>[14x]MAKELHFNKDMQALKRMQAGVDKLATVVGVTIGPKGRNVVLESKFGAPKIVNDGVTIAREVELSDPVENIGATLVRQAAARTNDTAGDGTTTATVLSAAFIAEGMKIVSAGTNPVQLVRGMEKTVQELVKELRKMSSVVQTDKDLANVACVSAGGNTDIGSLISDAMAKVGRTGVVTMEEGKTAEDQLVFVEGMQFERGYTSPYFVTDPERMICEYENCKILLVDKKISTARDIITILESAIRGNYPLLIMAEEVEQEALATLVVNKLRGTLKVVAIKAPGFGERRSSYLEDIAILTGGTVVRDEMGVSLEQATDAVLGTAAKITITKERTTVVGDGSTAADVAARVKQIRNLQMQTDQDYEREKLQERIARLSGGVAIIQVGAQTETELKEKKLRVEDALNATRAAVEEGVVPGGGCTLLRLSEKVDVIKRRMTDPEQQMGADIIKRALCYPIKLIAQNAGVNGSVVMNEVMKNLDRPHYGYNAATDSFENLMETGIIDPSKVVRCSMENAVSVAKTFLLADVVVTELKEIEAGAKPNPVAPGAAGFGGGL

Chloroplast chaperonin, consisting of multiple subunits, mediates folding of the highly abundant protein Rubisco with the assistance of co-chaperonins. Unlike homo-oligomeric GroEL and mitochondrial Hsp60, chloroplast chaperonin consists of multiple subunits, diverging into two distinct but related α and β types. Though the authentic chloroplast chaperonin consists of both subunit types in vivo, homo-oligomeric Cpn60β is functional in refolding model substrates with assistance from co-chaperonin in vitro. ATP hydrolysis drives the chaperonin allosteric cycle to assist substrate folding and promotes disassembly of chloroplast chaperonin.

The crystallization of functional hetero-oligomers of CPN60 did not succeed, whereas the crystallization of CPN60β1 homo-oligomers was achieved by the sandwich method. The crystals belong to space group P21, with 14 subunits per asymmetric unit. In our study, the first crystal structure of Chlamydomonas chloroplast chaperonin homo-oligomer (CPN60β1) was solved at 3.8 Å, and displayed a rigid body and structural features such as looser compaction, a larger central cavity, less contact sites, and an enlarged ATP binding pocket compared to GroEL. In overall architecture, CPN60β1 presents as a typical type I chaperonin, with a 7-fold symmetrical cylinder structure consisting of two stacked rings composed of seven subunits. Similar to GroEL subunits, each CPN60 subunit consists of an equatorial, intermediate, and apical domain. However, there are three features that distinguish the chloroplast chaperonin: (1) The central cavity of CPN60 is relatively large; analysis of helices H-I (aa residues 231–273, highlighted in Fig. 2b), which reside on the inner surface of the cavity and are involved in both binding polypeptides and interaction with co-chaperonin, revealed that the diameter of the central cavity of CPN60β1 oligomer is 6 Å larger than that of GroEL. (2) The structure of CPN60β1 is loosely compacted; a closer view revealed that the equatorial domain of CPN60β1 extends away from the central axis, with E1 (aa residues 2–136) and E2 (aa residues 410–525) domains rotating counterclockwise and clockwise, respectively, in comparison to the equatorial domain of GroEL, although the overall structures merged well. The number of amino acids involved in contacts in one CPN60β1 subunit is much less than that in one GroEL subunit, especially in the apical domain. (3) Finally, CPN60β1 resembles the allosteric intermediate state. The ATP binding pocket in CPN60β1 is wider, suggesting that adenosine may be more readily released. In CPN60β, positions 153 and 154 are occupied by glycine residues that have no side chains to aid closure of the ATP binding pocket upon co-chaperonin binding.>MISMKPRYKPDWESLREHTVPKWFDKAKFGIFIHWGIYSVPGWATPTGELGKVPMDAWFFQNPYAEWYENSLRIKESPTWEYHVKTYGENFEYEKFADLFTAEKWDPQEWADLFKKAGAKYVIPTTKHHDGFCLWGTKYTDFNSVKRGPKRDLVGDLAKAVREAGLRFGVYYSGGLDWRFTTEPIRYPEDLSYIRPNTYEYADYAYKQVMELVDLYLPDVLWNDMGWPEKGKEDLKYLFAYYYNKHPEGSVNDRWGVPHWDFKTAEYHVNYPGDL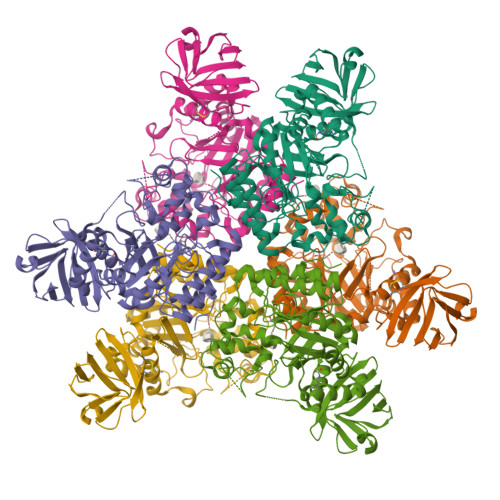PGYKWEFTRGIGLSFGYNRNEGPEHMLSVEQLVYTLVDVVSKGGNLLLNVGPKGDGTIPDLQKERLLGLGEWLRKYGDAIYGTSVWERCCAKTEDGTEIRFTRKCNRIFVIFLGIPTGEKIVIEDLNLSAGTVRHFLTGERLSFKNVGKNLEITVPKKLLETDSITLVLEAVEE[2x]>GASAQPLDVKIQEIWSRSANITWTAPYSGNSPITKYFVQYWKDKAGSQMLQEEEVTAAHSSVVINNLHPGTSYALTVIAENEIGHGEPSETVRFITGEEEPSGPPTDLWVESRGPFTILVRWKAPPKEYWHGKLKGYYVGYKMEGSPQPYSFKTVEAMNVNITHEYLLNSLKKSTKYSIVVKAYNAAGTGPASQELIVKTLDGVLPRPPSVSLLSASDSTISVKWGHTISRDEPVTGYTLHYRKKVGHWLHVPLLASDQTRYTLTGLDSDTTYNVYVTANNRYGRGDPSGILSVRTGD[2x]

Recently, a shortened Dscam (sDscam) gene family with tandemly arrayed 5′ cassettes in Chelicerata species has been identified, which encodes ∼50–100 isoforms. Chelicerata sDscams could be classified into two subfamilies, sDscamα and sDscamβ, containing one and two variable Ig domains, respectively. Crystal structures and cell aggregation assays demonstrated that both α and β subfamilies of sDscam used Ig1 for the isoform-specific trans recognition in a hand-in-hand manner. Furthermore, the cis interactions were established by the three FNIII domains of sDscam, which assemble into a cross fold with a kink between FNIII2 and FNIII3.

We evaluated the cis polymerization of sDscam FNIII domains on living cell surface and determined the crystal structure of sDscam homo cis-dimer. Thus, this kink conformation may reflect a physiological geometric assembly. The inter-domain interface of the kink contains a salt bridge formed by R404 and D578, and the hydrophobic interaction mediated by L492 and L496. The dimer interface buries 2109 Å2 of surface area, which is composed of one FNIII2-FNIII2 interface, two FNIII1-FNIII2 interfaces and two FNIII1-FNIII3 interfaces. Consistent with our cellular data, FNIII2 played a pivotal role in sDscam cis recognition as it formed intermolecular interactions with FNIII1 and FNIII2 of the other protomer and intramolecular interactions with FNIII3 of the same protomer. The FNIII2-FNIII2 interface was located at the center of the cis homodimer, where P395, P417 and Y420 formed a hydrophobic core. Y420 appeared to be essential because it formed a hydrogen bond with P395 and π–π interactions with the symmetry-related Y420. The FNIII1-FNIII2 interface was dominated by hydrogen bond networks formed by the side-chain of N357 and Q485, and the main-chain of L358 and E486. In contrast, the FNIII1-FNIII3 interface was composed of both hydrophobic and hydrophilic interactions. To verify the cis-dimer interfaces, we made single-site mutations on the FNIII1-FNIII2 interface (N357A and Q485A) and the FNIII2-FNIII2 interface (Y420A). Evaluated by the cKIT tyrosine phosphorylation assay, all the mutants significantly reduced the cis-interaction.> XRMKQI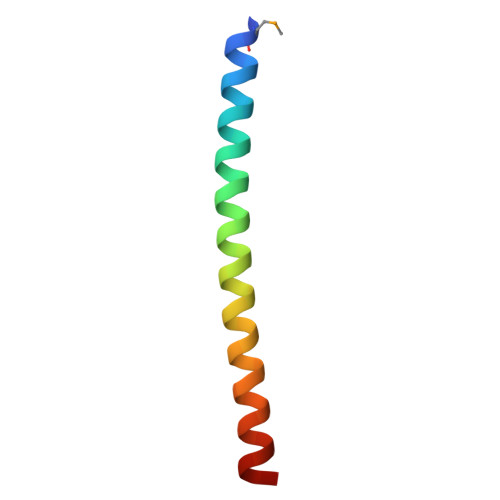EDKIEEIESKQKKIENEIARIKKLLQLTVWGIKQLRARILX3-{2,6,8-TRIOXO-9-[(2S,3S,4R)-2,3,4,5-TETRAHYDROXYPENTYL]-1,2,3,6,8,9-HEXAHYDRO-7H-PURIN-7-YL}PROPYL DIHYDROGEN PHOSPHATE | C13 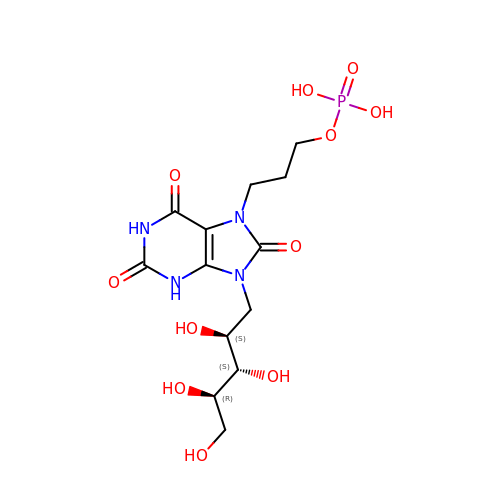H21 N4 O11 P | KPHFGOGGKPGLTM-OOZYFLPDSA-N>MASLRSRCDQLEERVSAAEDEINEIKREGKFREKRIKRNEQSLQEIWDYVKRPNLRLIGVPESDVENGTKLENTLQDIIQENFPNLARQANVQIQEIQRTPQRYSSRRATPRHIIVRFTKVEMKEKMLRAAREKGRVTLKGKPIRLTVDLSAETLQARREWGPIFNILKEKNFQPRISYPAKLSFISEGEIKYFIDKQMLRDFVTTRPALKELLKEALNMERNHHH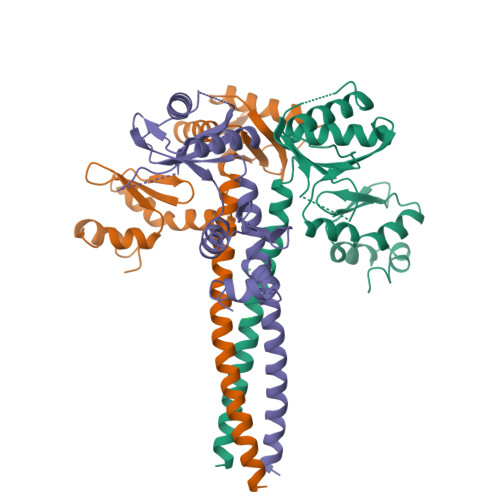HHH[3x]>[2x]HHHH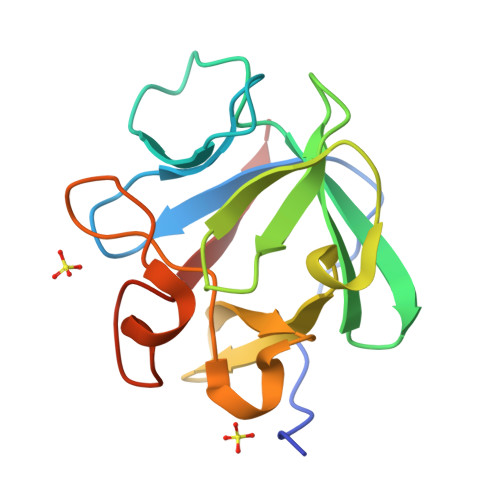HHFNLPPGNYKKPKLLYCSNGGHFLRILPDGTVDGTRDRSDQHIQLQLSAESNGEVYIKSTETGQYLAMDTDGLLYGSQTPNEECLFLERLEENHYNTYISKKHAEKNWFVGLKKNGSCKRGPRTHYGQKAILFLPLPVSSD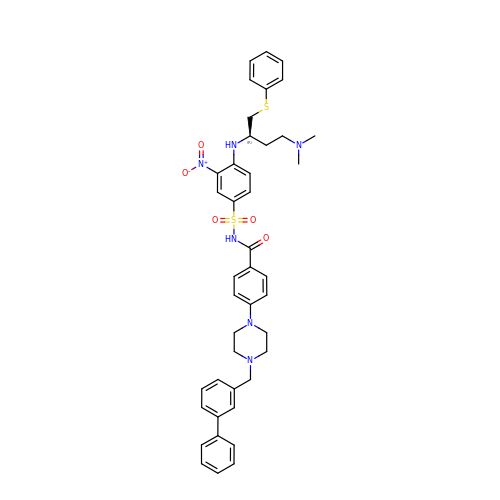4-[4-(biphenyl-3-ylmethyl)piperazin-1-yl]-N-{[4-({(1R)-3-(dimethylamino)-1-[(phenylsulfanyl)methyl]propyl}amino)-3-nitrophenyl]sulfonyl}benzamide | C42 H46 N6 O5 S2 | YVZYKXDSCCZVEP-PSXMRANNSA-N> ATFISVQLKKTSEVDLAKPLVKFIQQTYPSGGEEQAQYCRAAEELSKLRRAAVGRPLDKHEGALETLLRYYDQICSIEPKFPFSENQICLTFTWKDAFDKGSLFGGSVKLALASLGYEKSCVLFNCAALASQIAAEQNLDNDEGLKIAAKHYQFASGAFLHIKETVLSALSREPTVDISPDTVGTLSLIMLAQAQEVFFLKATRDKMKDAIIAKLANQAADYFGDAFKQCQYKDTLPKEVFPVLAAKHCIMQANAEYHQSILAKQQYYFGEEIARLQHAAELIKTVASRYDEYVNVKDFSDKINRALAAAKKDNDFIYHDRVPDLKDLDPIGKATLVKSTPVNVPISQKFTDLFEKMVPVSVQQSLAAYNQRKADLVNRSIAQMREATTLANGVLASLNLPAAIEDVSGDTVPQSILTKSRSVIEQGGIQTVDQLIKELPELLQRNREILDESLRLLDEEEATDNDLRAKFKERWQRTPSNELYKPLRAEGTNFRTVLDKAVQADGQVKECYQSHRDTIVLLCKPEPELNAAIPSANPAKTMQGSE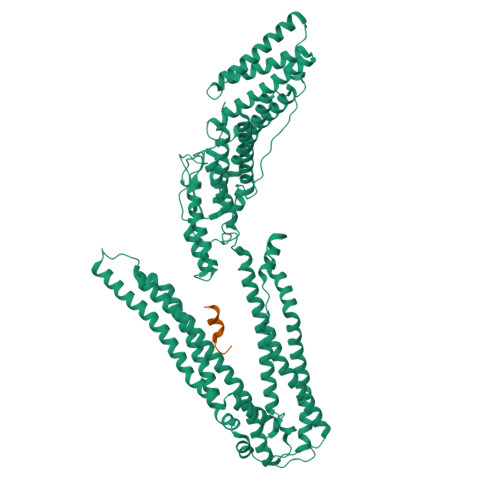VVNVLKSLLSNLDEVKKEREGLENDLKSVNFDMTSKFLTALAQDGVINEEALSVTELDRVYGGLTTKVQESLKKQEGLLKNIQVSHQEFSKMKQSNNEANLREEVLKNLATAYDNFVELVANLKEGTKFYNELTEILVRFQNKCSDIVFAR;> ELYPLASLRSL> MRRTVRALYNSFERGWKDKTVHPLDRRGRFNLDEAAAELQLDEAYVASLYKPLHYTYSMKGQRYPAEQGRTSRPGSLAASRDRMFPLYRRNYKLNR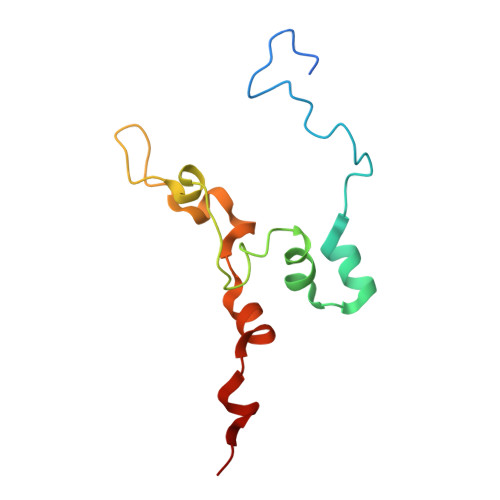ELRVLDHRRISTD methyl 3-(4-oxo-4,5-dihydrofuro[3,2-c]pyridin-2-yl)benzoate | C15 H11 N O4 | 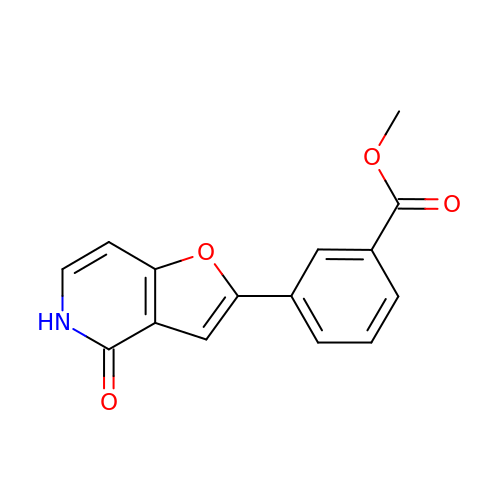OVTGPKXYLOQTEQ-UHFFFAOYSA-N> MAASSPLVRLRRLALPLALVVLCAAAAHGQTLSSAVLTASNTIMATLSNVTTSTDCRAAFAYFDSNNATKAASPFANCTVSGTTSVTLILASGVSYAAGDQLNIKVNQTTLNTTAGVPFVPAAAAAAVQPVLGAATLTTASSLVVKLPLSSGNTMPDGYATNMTICGAAVQLLSAAGAVKASPFSACLLAADTLTLTLTSSGTYAPGDVVNVVAGQSTLKNGATSYTKSAAGSVIRPTLTTVSLATTTTILIGASAPVSLPANASADVCNSIFTVALKSGTALPTALSACMAGPAVTAITATFANGTTYSDGLTVTIKANQTLLRTGDQSASSPLFLPPASALVIAPTVLSASLTSATSITVQLPVSSTASGTLDAAGCNGAFELRAAGSSASKSSPFSACALASNNTALVLTLASASTYTAGDIFNVKSGQSLLQVGSTAYVPQAVSVLPTLSTAILVAASVVRVGLPVVSSIPAPYSADDCARSVIIAAANSTAAKAISGCVLSADGKALLVTLGAAYAAGDTVNVRTGQWQLRAGASVTLGPNYIAASTPVAIVPGFSSAVLTSATQVTVQLPLASALPATISASECGDAFDLLDASGTTSRVSPWTGCSIGSNNTLVLNMTAGIYVVGDQVTPKSGQTKLTFANTTAYGVLLTPINPILTAATTAMLTASSTIVVALPYAANLPASTNNGTVCNAAFDLVSAAGASRTAPFSACSISGGTTLTLTIASTASYTAGDRINVKSGNSAFLGSLSASGPAFVHAGTAIVITPTVVSTALISNTNVFVSLSAPTSASAFNQSICNGAFDVSGLATPFTNCTLSADGTGISFLLASAGSVTSGVTTINVKSSQLFLLAAGSGSSDSPAFVPRGSALTISEAKLAGAYLTAANTIIVKLSVAAAAVDGFSSSCNNVFTLFNSSGTARASPFSACTLSTDGLTVTLTTSSWVSTDKLNIRSDQTLLKVLGAANGPSYPALSSATEVSPAITSAHITSPTTIIVPLPVASDLTGSSCSFLVLTAATSNCALSNNGTLLTVTLSGSYTIGDTININALNSALRGTSSTGALYQPVSGATAATIQPTIGAVQVTTSTRLLVTLPAAMSSPVPNPLTADACNAALDLSGKSSPFAACTASGTTLTLDLASAFVPGDRLNVKSTNTALRLGTGASALFFQPLATSPANILNPTFVSAKATSTSVVVVSLPAASTFVKSGSATAGLVKADCDTVLAMSSGSLVGSGNACDLNTTSSSQLIVTLAGTTYAPGQTINVLTTNTMLLAGSSSGPAYQPRTITINPAYLSSDVVATAPDTVVVTLPVTSGLFAADGSSLGSTLTAAQCATVLEVKAGTTAKGLASCSLAGTTLTVKLLGNNSDVYTGGDTFNFKDTNALLLAGSANTAPAYKALATAAVIVPNLYKAVASAGDTILITLPAASTFVVSGSAVLSVSDTVCNTILTFTNSKTVKSGTNCVITGAVLSLTLNSAITDQTTVTINSGGQTTLVSGTGTTGPAYKAGTAAPISPAYLTSAAARSATSIVVTLPFTSTVNGATLTKATCDTIVEVLNGGDATKPRTLDSGTPCTLATTLLTVNLAATESFAPGDTVRIKSGNTVLLIGSAGGNAPYVQATTATPIALGYVTSSIATKATEIKVTLPVPITLIKAGVSVASLDKTDCDTLLTVASGTLAATGSCALSGTVLTITTTSTYTPGTTTVQFTAVASSASVKILGGAGTTGTIIAALSAASSVLPGYLTSAVISGANTFTLTLPYAVTSGGNPTCSDIIEIKAANGAMKTFNGVCSVASATTVTGTTNEALLASDTVTLKGAQNALTTTTGSKIYAATAAINIQPAYLTGAYAIDDKKFVVVLPYASTLAAGTCSSIVSVTDNNNGPAESGCSLALDGTGIYLTVTVSASLTATAWKVDFKAAQTALTVGSTAWAPMATGTAKSLNAGATTWGSSIMTATAVATNVLEVTLPMSSYMADISSGCSPVTFSTANTAASCKLIGTTSSPNSILQITLTAGYVAGAVSLANAAGLIKAGSASGTAIGAASTVTIKPTFVSAVATGPRTIVVALPIQSKIIKGAPTCTGGAVTCSSGTATCQSGSPACSAAGTYTCTATDPTVGLTCAAPTVTCPASTTAACITGGSPGSIATAGNGPGCAAATTDGGTAACGAGISAVCYSSSLTTAARCASGSAFSAANGNNCDDSASSIDLDPTCYTSSTMTATAVSDAALCTGWISGMPTCSSSGKFACVSATGPTCTASTAPTCKSPFTGTANCAITFSCGGTGLVVPTCTGSFTGCSKGTTGDTCDDDIASPADCSTIFSLTGGTATIAGCSNPGSDFTAPYTTTVTLATANWVPGTTLSVAADQAAAAATNYLKPTAAITLLYTTKPSGAVVIYPSISSATLTGPKSLQVTLPVAASVPSSGLSPADCNNIFQLYATGTTTPKTAAVFSACYLGADKQTFYLTLAAAAASTTNANTYAVKDLINIKAGQSLLKADSATAANRLAFAPLPDALLIRPAITSAVATTIASAAVIKMQLPLTSNLGTVNCATTGIKVRVDDATDKTQANTGACSISSDANGAVLTLTLNQALGASDFTTGKGVSVVVVATSSADATKLQLFGGSDNTGPLYVTGSIPVYDVVTPGQSIVSAKAIASNQVEIKLPAPSTITTGNTCANFLAFTPTRTISSCVYDAETQLVTATVDQFAAGDAVNIAGAPNLLKYATAAATLTDYAALAAAATVSPALVSAYTVDSTTIAVVLPATSSFYSGATNSATKVASLTDVECADVLTVLLAGKTNSAGVSACATPSNCRTLFSGAACLLGTTSAGDTLLTIKLGASYAAGDAVDVWDKNAGLNGATAAAKPLRVGTNVQALYVPRRMPVVIEPRIVSASATGARTIAVTLPVTSQLIDSTGTVISAPTQQQCASLVALPAGKSVASCAISSDFLTLTLTLAADFAPGDTVNIASGQTLLRAWKSDVGPGYELSGPLYTPSASAVTVTLSFFVSATSTAANTIVVTLPFPVKMYDLAASPAEILAADGATPTKDNCDSV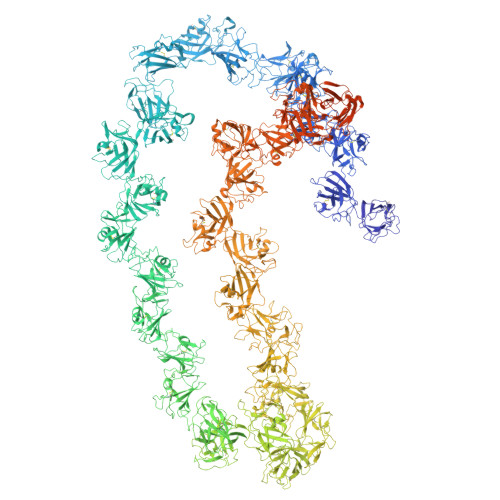IRVIPSGSTIARTLVAPGAGVAPCVLSGSGTTITLTLDTTVSSYATGDRIDVGFGNSANLRGAATAAAVANTSPKYTTVATLNAAASAAVVTIGPSIVSAAAASPTQVKVTLSATGTITTTPATVDDCNKIVTFTPAKTLAATSPCSVAGTTLTVNLDKATPYAGTDAVNIAAANSLAATTNPLKAGSLAFVAKATAVTIDPNLYTATAIDSLVYEVALPAASSVGSTALTAAQCGAILSLTGGRTISSTVTAPCVLDTTKTLLTVSLGTAYADGDTVTLQSTQATPWLRAASDTGPAYKVGSTLIVKPTIASAKATTATTIEVTLPVTSVIWSTSGGAAVSTALTATECGKILSVKRGSGTVALSASGACSLSSSGSTTLTVTLASDQVFQAGDKINILASNTDSANTDKYLVATTSSSGQAYIARSSDVVIAPGFINAAYAVGPNTLSVALPVVSSIATDNDCSTVVTVRASATPTTTRTVSGACTVASDATGYYLVVTLAAGTPFVSGDEVLIKSGNTALVGSIAYASGAAGATKPIYANFDDAILTAPTTVLVTMAAVTTVSFTSKADCDAVFVFSGAGNTTKTTSPIASCALAPDGLSVTITLSSADAYVPGDAINVVKDQTSAKVGGVGGTNLVPYPTATTISPRPFGAKATLVAPTSVAFSLPAVSSLPAATAAADCNAAVRYTDVAGVDAVNPFTSCALTPDTKGVVLNTASPIYKAGDVMNIKSGNAAVRWGPQASGAAYYPAAADVPVFATVATATLVDPSTVVLNLPTVSAIPDNFTVPDCLRAIEFKTAAGVTKNGTVASCMLMPDRLGLQVKLLSAGNFSAGDTVNIKPEQAELRSSALATGPSYVPKLAAQVVNPALFANANLTSATAITVRLPFASALATGADCKAVLALLGAGGVAKNVSSCSLGADGVTLAVTIPAASFVGGDVLNIVPGQRALTLADGTTAYVPSKAGVLVTPNIVSATLTNATIVTVALPTASVLTSTAAADCNAAVVIARNGSAVASPLSACAVSADGLSLTLTAAATYKPMAGDTVDVAVSQTVLRAGSATGPAYVPRPSPALITVPSPPPSPPPSPAPSPPPSPPLSTANYSARGLATGPLSCNVLIGDLTVTTTAGNFTTIGMASYAGKDASYKGSCKDAVTGAVYTDDTVASTLPAGLTGLVLSPVTALASVWDLKSVADLANTNKDYLRLFGVPVNASAYGTAVQLLAYDYYVKGFVALETPAVAVLNVEGMVAANLLMYTKFFDGLNTSVAGRDITAAQALAAGQYALAAVLEDSIAPINTTDPASILALLNVTYSVLTANATSAAGRRLLQTAPAPFTQLQAQATALAAAAAGSNALVAAQQARLITAINAGTSISAAELTNIINEASKVIVAQSTVIATAATGLGSGAISPASFTSSYTGSALSTLVAQQQLAATPGSDVTAGPAPSPPSDKKKSNTGLIVGLVVGLVGGAIVITLIVVFIVMRRRKQNVAAAGQATA> MTISMLVSSVLPGTVVDDLAYAELYSDPPGLVPLPEEEPLIAKSVAKRRNEFITVRHCARVALGDLGVPPVP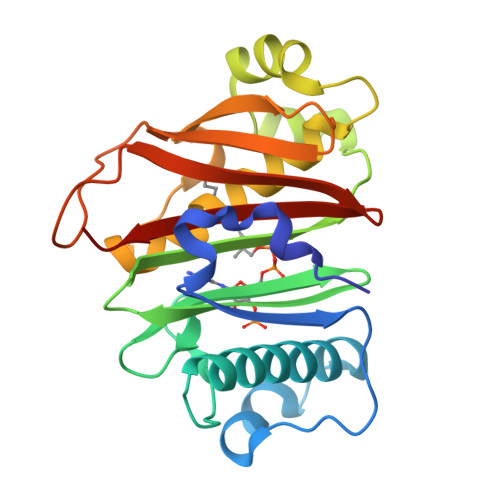ILKGDKGQPCWPDGVVGSLTHCSGYRGAVVGRSAAVRSVGIDAEPHDVLSNGVLDAISLPEERDEIPSAMPDGLHWDRILFCAKEATYKVWFPLTNRWLGFEDAHITFEADDSGRTGRFVSRILIDPSALWGPPLTTLHGRWSVERGLVLTAIVLLEHHHHHH> MNKLAITVLLCFFPALALAENGALSFAPPASDLSVVFLGNLFGVVDGVLHGTGSQIMGNMFGVFNSAVLALGGIIIMYTLMVSTMNTAHEGQMLGQKWSSIWIPLRSTFGLALLIPKASGYCMMQVFFMWVIVQGVGAADKIWEAALSYLNRGGVIIQAQADPTKSLQAAGSSSSGVAKGALTILGGQICMLGLQKQLQAQRDLYLSQSKSPPCGGNPTPEMNTFCRTAIPDFISTVNFVKKQNDDTPKDLTANQPASFELDMPNFDKSSPFYFLNGICGTVKWNNISALNSTNQSDNKGLVTVGGAGSNSSMGANSLNITSSQLQTARLSRAIAIQQMYVTLSTVAQVMVNNDPAFSTTTSTGNSKNDFSAIAKQQFGVPYKSSGEVCTEYQQVCQTWGSVPSSTGSTTGVLFNGTEFLGAINDYNGIMMPTL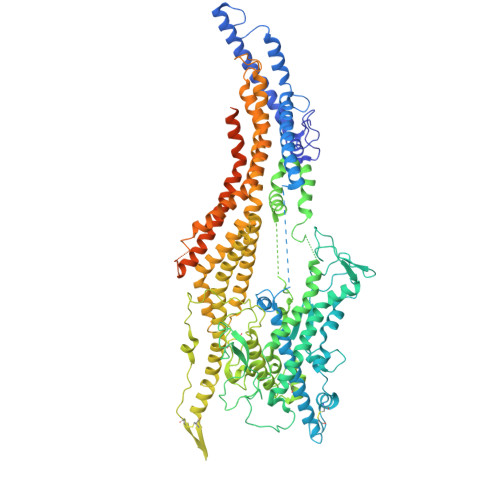NLIRQATSKEFDKKSRDFIAEANAKGWIMAGSYFFDLVKLNGSATEFADQFDTGTGLDKSSFDPTQLTKPFGKTCQDPYSLLCTWFQNKSDKLIQIQSLIDGVPALGQDGVKQPDLSDNPQRQSVSGPLSSTVYGFVNNSMMVQLPGQPGIKPLTFANLINFKVDTSLYYMKHQDFDCGRVKILFFSFCLGRMMGDLFYNYVFRYVYNFFLAIFGEMINSIVMAFLMIPLQGMKDIFIVGVQTLTQPGINPIVALANMGTMYINFSGTLWLTLLNMAVVSSLIPLFGIFIFALIMMAMPLLMAWIGTMVSIGFVTAYYIPVLPYMIFTFGSFAWLIAVIEAMVAAPIVALGVTHPEGNEAFGKGEFAIMILVNVFLRPSLMIIGYIAAIALSYVGVWILNAGFDHAISYIQSDQGIETWEKGTSSNDAKRFFQSAGNWTGAKMDTSQWDNFKDKLTGDYQSTALEGGYTGWAGVYAFFFSILIYTSMYLIIVQKAFTLIAHLPDKVLRWIGGSPESFGQETMQWGEEAKGRVEKAGEATYGAEKAIGDKLGAKGQEMLGKLGPQAKKISENAGDVSGKGKNSGGSQTGPSSKPDTGQQLGGSDSGTPTSTPPPE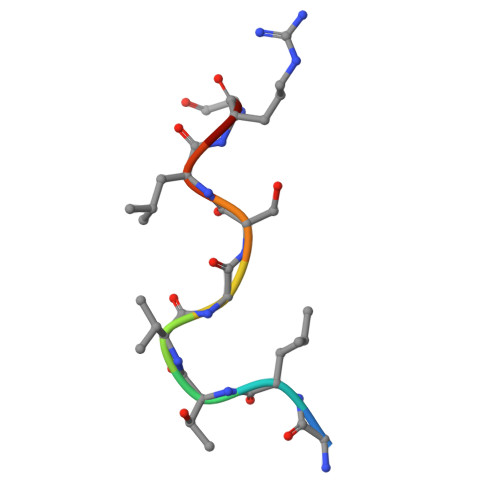> GLTVGSLRG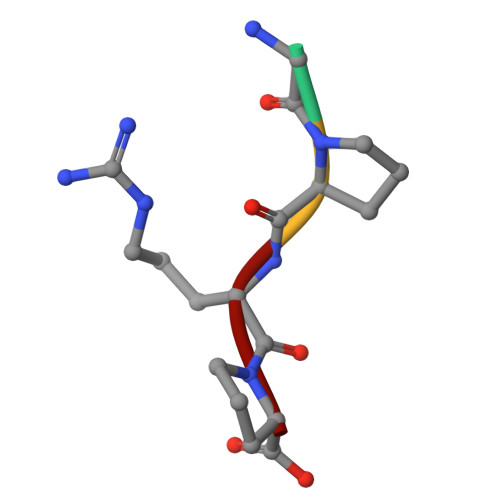> GPRP>[2x]GGFDYDVVVVGGGFAGATAARECGLQGYRTLLLEARSRLGGRTFTSRFAGQEIEFGGAWVHWLQPHVWAEMQRYGLGVVEDPLTNLDKTLIMYNDGSVESISPDEFGKNIRIAFEKLCHDAWEVFPRPHEPMFTERARELDKSSVL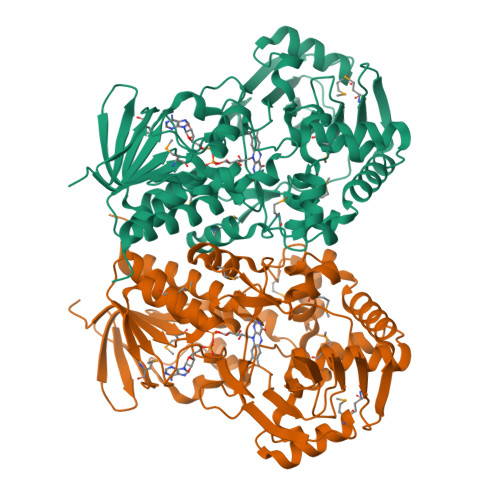DRIKTLGLSRLQQAQINSYMALYAGETTDKFGLPGVLKLFACGGWNYDAFMDTETHYRIQGGTIGLINAMLTDSGAEVRMSVPVTAVEQVNGGVKIKTDDDEIITAGVVVMTVPLNTYKHIGFTPALSKGKQRFIKEGQLSKGAKLYVHVKQNLGRVFAFADEQQPLNWVQTHDYSDELGTILSITIARKETIDVNDRDAVTREVQKMFPGVEVLGTAAYDWTADPFSLGAWAAYGVGQLSRLKDLQAAEGRILFAGAETSNGWHANIDGAVESGLRAGREVKQLLSLEH2,2,3,3,4,4,5,5,6,6,7,7-dodecakis(fluoranyl)-~{N}-oxidanyl-~{N}'-phenyl-octanediamide 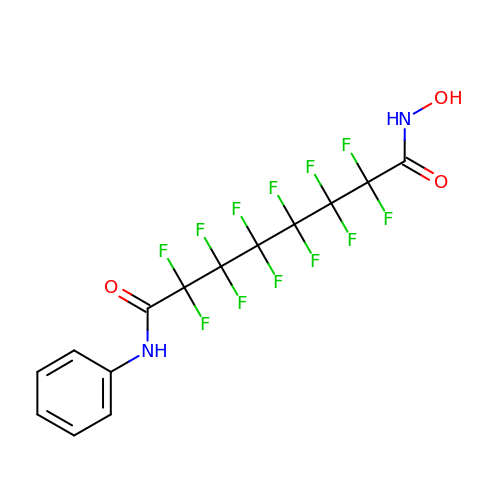| C14 H8 F12 N2 O3 | PVEUUUJZCFCCIZ-UHFFFAOYSA-N>MLNVGATAPDFTLRDQNQQLVTLRGYRGA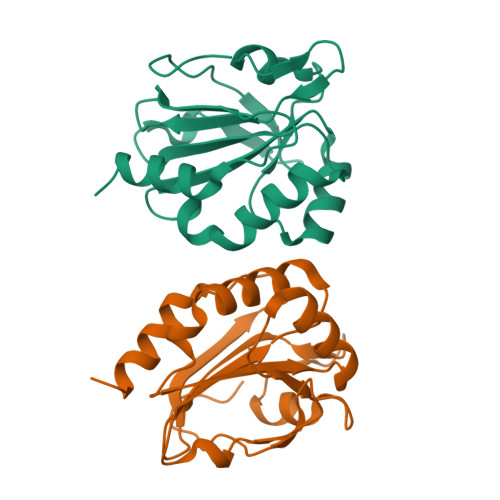KNVLLVFFPLAFTGICQGELDQLRDHLPEFENDDSAALAISVGPPPTHKIWATQSGFTFPLLSDFWPHGAVSQAYGVFNEQAGIANRGTFVVDRSGIIRFAEMKQPGEVRDQRLWTDALAALTA[4x]>MSIEKVPILGKETIHVGYGIADHIVREVIANLASSTYVIVTDTNMARTPQYSKLTDDFKTNLSEKRPESRLLTYCVSPGENNKNRATKAAVEDFLLQQGCTRDTVILAVGGGVIGDMIGFVAATFMRGVRVVQVPTTLLAMVDSSVGGKTAIDTPLGKNFIGAFHQPEYVFCDVSFLETLPARQFINGMAEVVKTAAIWNEEEFTRLENFSKKFLSVVTSKKPDLQSIKAELVKTVLESVRVKAGVVSSDEKEAGLRNLLNFGHTIGHAIEAVLTPEALHGECVSIGMIKEAELSRYLGILPPVAVARLSKCLVAYGLPVSIDDKEFLKKVGPKRHYVEIDILLKKMAIDKKNDGSKIRCVLLEKIGKCYQLKAHQVSKQDLSFVLTDEVLVHPFTNPPKENIIVPPGSKSISNRALILAALGNGTVRVKNLLHSDDTKHMLDAVASLKGAEISTEDNGETIVVKGNGGNLVTSGEELYLGNAGTASRFLTTVASLVGKSQASDDVILTGNARMQERPIGPLVDALGSNGSEIEYLNKQGSLPLKISAGNGLKGGRIELAATISSQYVSSILMCAPYAKEPVTLALVGGKPISQLYIDMTCAMMKSFGIEVTKSTTEEYTYHIPKGTYKNPSEYVIESDASSATYPLAFAAMTGTSCTIPNIGSSSLQGDAKFAVDVLKPMGCKVEQTTTSTTVTGPPRGHLKPLPHVDMEPMTDAFLTASVVAAVAKGGSSTSITGIANQRVKECNRIEAMVTELAKFGVPANELPDGIEIHGIDIEDLKTPEISKRGVSSYDDHRVAMSFSLLAGLCKEPVLILERSTTGKTWPGWWDILHSKFKIELDGYEPPFNTDKHVDKSSDKSIIVIGMRGTGKSTLSEWLASFLGFKMLDMDKYLEEKLGTGIKSLIKAKGWEYFRQEEAIVAKECFTKFSKGYVLSTGGGIVEGEDARQQLKSYADNGGIVLHLHRDLDETVTFLAADTTRPAYSSEVQEVWLRREKWYHECSNYHFYSSHCSTEDEFNHLRRSFVNYIKLITGAERPVVPAGRSAAVVLTSPDLNEVVGDLESITIGADAVELRVDLFKDTSAEFVAAQIAVIRKHADLPIIYTVRTVSQGGKFPDENVDELKSLLLLGIRLGVAYVDLQLTAPNELIEEISSKKGFTRVIGTYQDINGELKWNNVEWKNKYNQGVSMNADIVRLVGKANSIQDNLDLENFKKQNTLKPLIAFNLGSQGKLSQVLNGTFTPISHKLLPNDEEFLTIGELNQTYFDIGGFTAKKFWVIGSPIEHSRSPNLHNAGYKALNLPYQFGRFEATDVDVVYDNLINKPDFGGLAITMPLKLDIMKFATKLSDAAETIGAVNTLIPIEGGYFGDNTDWVGISNSFIRAGVPPKSSSNGLVVGAGGTSRAAIYALHQMGCAKIYLVNRTAAKLEELVKSFPKDYNLEIVETEQQADKASKVSLAVSCIPADKPLDGEVLKKIERILSNGSEQSAGFKPTLLEASYKPRVTPIMKLTEEQYKWKVIPGVEMLVNQGDRQFKLHTGFTAPYEIIHRAVVEE[2x]

In the human fungal pathogen Candida albicans, ARO1 encodes an essential multi-enzyme that catalyses consecutive steps in the shikimate pathway for biosynthesis of chorismate, a precursor to folate and the aromatic amino acids. In Fungi and Apicomplexa, the second to the sixth steps of the shikimate pathway are supported by five enzymatic domains combined in a single protein known as Aro1 or AroM. Aro1 forms a flexible dimer allowing relative autonomy of enzymatic function of the individual domains. Our activity and in cellulo data suggest that only four of Aro1’s enzymatic domains are functional and essential for viability of C. albicans, whereas the 3-dehydroquinate dehydratase (DHQase) domain is inactive because of active site substitutions.

Although we were unable to obtain crystals of C. albicans Aro1, we used cryogenic electron microscopy single particle reconstruction (cryoEM SPR) to investigate the Aro1 structure. Nevertheless, we were able to identify a subgroup of particles corresponding to dimers of full-length Aro1. After 3D classification, we identified 87,484 particles belonging to a stable conformation representing a dimer of full-length Aro1 at resolution of 4.19 Å. In this map, we performed only a rigid body fit of two high-resolution models for Aro1DHQS-EPSPS and Aro1SK-DHQase-DHSD domains. As implied by the crystal structure of isolated Aro1DHQS, dimerization of the full-length cryoEM SPR structure of Aro1 is mediated by extensive contacts between the Aro1DHQS domain, resulting in an arrangement similar to the one observed in C. thermophilum AroM homodimer. Notably, we did not add any ligands to C. albicans Aro1 sample used for our cryo-EM analysis, nor did we observe any evidence of endogenous ligands in the five active sites, in contrast to the crystal structure of C. thermophilum Aro1 that contained numerous ligands. Interestingly, within the Aro1 dimer we observed asymmetry between the monomers, with the Aro1SK-DHQase-DHSD region tilting ∼55° relative to the Aro1DHQS and Aro1EPSPS domains. The Aro1SK-DHQase-DHSD region of subunit 1 is tilted away from the Aro1DHQS-EPSPS region and is referred to as the “loose” monomer, whereas the Aro1SK-DHQase-DHSD region of subunit 2 is nearly parallel to the Aro1DHQS-EPSPS region and is referred to as the “tight” monomer. The Aro1DHQS domain, Aro1EPSPS subdomain II, and Aro1SK-DHQase-DHSD backbones show nearly identical conformation within the core structure of each region with minor differences seen in some loop regions. This implies that the large movement of the Aro1SK-DHQase-DHSD region does not drive structural changes that modulate substrate binding or catalysis, but instead reorients and repositions the domains. However, each individual active site is more than 40 Å from each other and each face outwards from the core of the dimer.> KDNIRHGVCWIYYPDGGSLVGEVNEDGEMTGEKIAYVYPDERTALYGKFIDGEMIEGKLATLMSTEEGRPHFELMPGNSVYHFDKSTSSCISTNALLPDPYESERVYVAESLISSAGEGLFSKVAVGPNTVMSFYNGVRITHQEVDSRDWALNGNTLSLDEETVIDVPEPYNHVSKYCASLGHK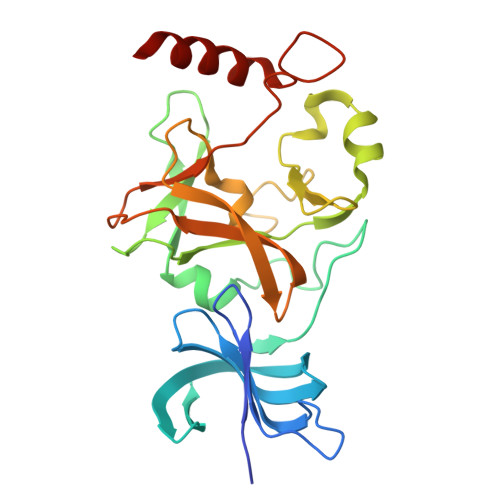ANHSFTPNCIYDMFVHPRFGPIKCIRTLRAVEADEELTVAYGYDHSPPGKSGPEAPEWYQVELKAFQATQQK> MHHHHHHMTMDEQQPQAVTPVYVGGFLAR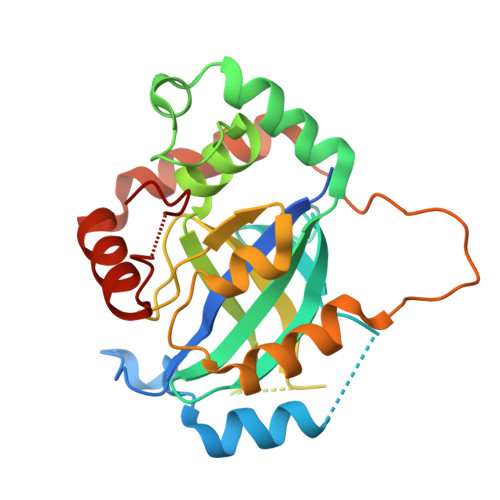YDQSPDEAELLLPRDVVEHWLHAQGQGQPSLSVALPLNINHDDTAVVGHVAAMQSVRDGLFCLGCVTSPRFLEIVRRASEKSELVSRGPVSPLQPDKVVEFLSGSYAGLSLSSRRCDDVEQATSLSGSETTPFKHVALCSVGRRRGTLAVYGRDPEWVTQRFPDLTAADRDGLRAQWQRCGSTAVDASGDPFRSDSYGLLGNSVDALYIRERLPKLRYDKQLVGVTERESYVKA> NLAA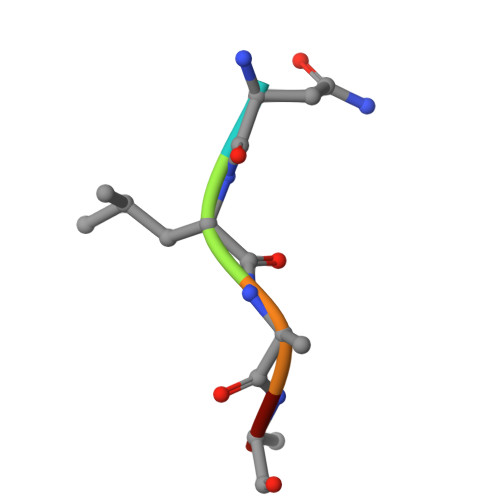R(2,4-DICHLOROPHENOXY)ACETIC ACID | C8 H6 Cl2 O3 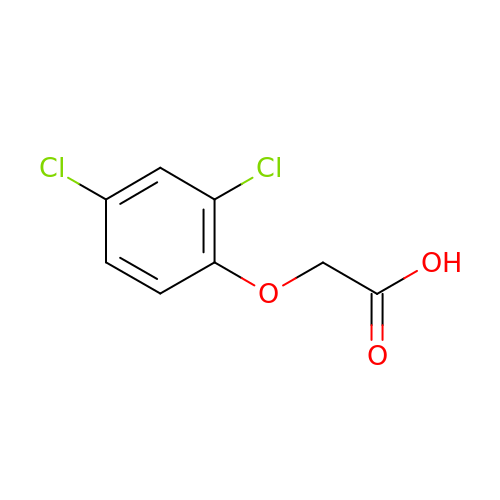| OVSKIKFHRZPJSS-UHFFFAOYSA-N> MRGSHHHHHHGSGSGSGIEGRADNATTIKIATV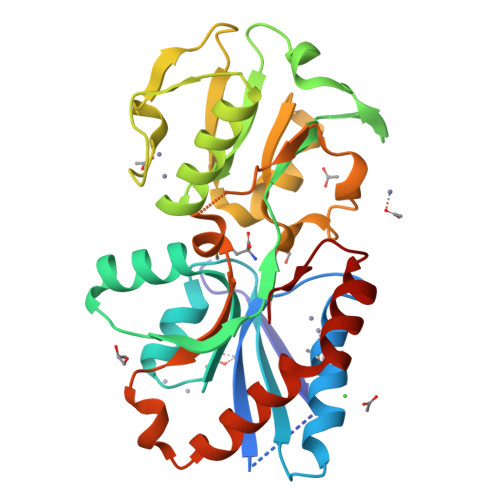NRSGSEEKRWDKIQELVKKDGITLEFTEFTDYSQPNKATADGEVDLNAFQHYNFLNNWNKENGKDLVAIADTYISPIRLYSGLNGSANKYTKVEDIPANGEIAVPNDATNESRALYLLQSAGLIKLDVSGTALATVANIKENPKNLKITELDASQTARSLSSVDAAVVNNTFVTEAKLDYKKSLFKEQADENSKQWYNIIVAKKDWETSPKADAIKKVIAAYHTDDVKKVIEESSDGLDQPVW> GAGCAGACCAGA;> CGGCACTCA;>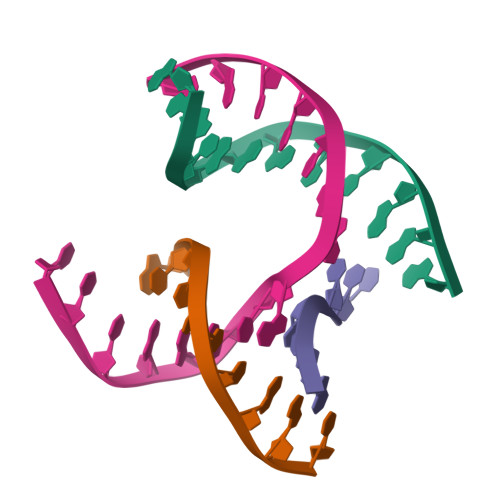 TCTCCG;> TCTGAGTGGGTCTGC Here, we present single-crystal X-ray structures of CheY from Pyrococcus horikoshii (PhCheY) in two different crystal forms, and the protein purification, crystallization and X-ray data collection of CheF (PhCheF). CheA autophosphorylates and subsequently donates the phosphate to CheY, yielding phosphorylated CheY (CheY-P; Garrity & Ordal, 1997; Bischoff et al., 1993; Rudolph & Oesterhelt, 1995; Rudolph et al., 1995). The concentration of CheY-P determines the switching frequency of the flagellum or archaellum, respectively. We observe PhCheY to have a domain-swapped, pseudo-dimeric fold, which may reflect inherent properties of the protein fold but is not likely to be of physiological relevance.

In striking contrast to all of the known CheY structures, PhCheY adopts an open conformation in both crystal forms, with the two subdomains of a given subunit directed away from one another. In both of the two PhCheY structures solved in this study, two polypeptide chains assemble by pairing the N-terminal subdomain of a chain with the C-terminal subdomain of the other chain; i.e. the α3/β4/α4/β5/α5 part of the fold of each subunit packs with the β1/α1/β2/α2 part of the other subunit [Fig. 1(a)]. The crystal form with space group P2 contains three non­crystallographic symmetry (NCS) molecules in the asymmetric unit. Superposition of the three subunits shows differing orientations between the domains, leading to an inter-domain movement of up to 90° [Fig. 1(b)]. T. maritima CheY and PhCheY superimpose well, with the main deviation in the connecting region composed of the short helical segment of the β3–α3 loop. This region is unwound in the PhCheY structure (residues 54–60) [Fig. 1(c)], facilitating the inter-domain movement. In all cases, the rotational movement of the C-terminal domain was calculated after the initial superposition of the N-terminal domain. The connecting region between the β3–α3 loop is partially disordered for the two subunits C and E. For both crystal forms an unambiguous trace of the electron density in the β3–α3 loop was verified by a feature-enhanced map (FEM; Afonine et al., 2015; shown in Supplementary Fig. S2 for the P2 crystal form). Owing to a putative cold-induced destabilization of PhCheY (P. horikoshii grows at 98°C), and putatively further induced by the crystallization conditions, the PhCheY fold disassembles into an open subdomain-dissociated conformation. At the high protein concentration in the crystallization drop, PhCheY can then reassemble from this open state with a partner polypeptide to form a domain-swapped dimeric assembly that is eventually removed from the monomer–dimer equilibrium by crystallization.

>MARVLVVDDAAFMRMLLKKILTQAGHEVVGEASNGKEAVEKYKQLKPDLVTMDIVMPEMDGITAVKEIMKIDPNAKIIMITAVGQEAKVMEALKSGAKGYIVKPFQAQKVIEEVNRVLSS[3x]>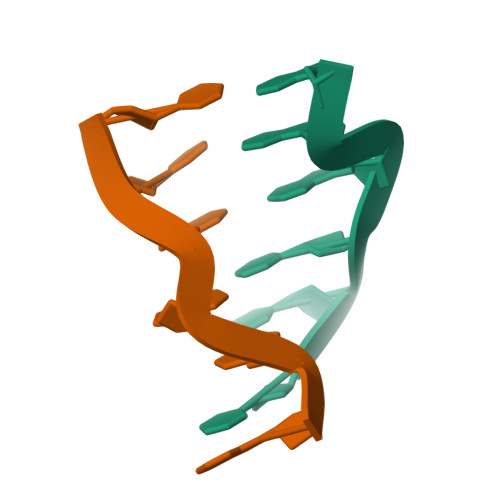[2x]CCCGGG> DNTTCDG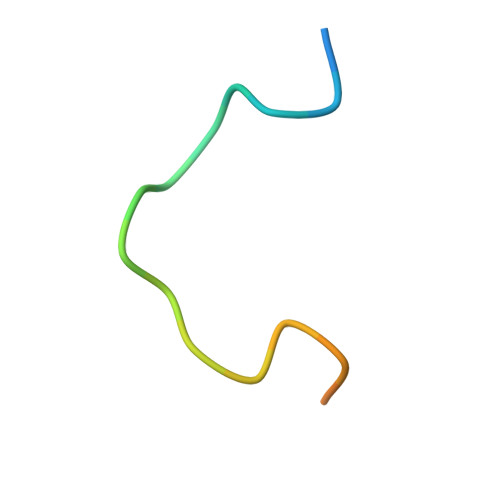PCGVRFRQNRQGGVR>[7x]SMHTQSQTVTVDQQEILNRANEVEAPMADPPTDVPITPCELTAAKNAAQQLVLSADNMREYLAAGAKERQRLATSLRNAAKAYGEVDEEAATALDNDGEGTVQAESAGAVGGDSSAELTDTPRVATAGEPNFMDLKEAARKLETGDQGASLAHFADGWNTFNLTLQGDVKRFRGFDNWEGDAATACEASLDQQRQWILHMAKLSAAMAKQAQYVAQLHVWARR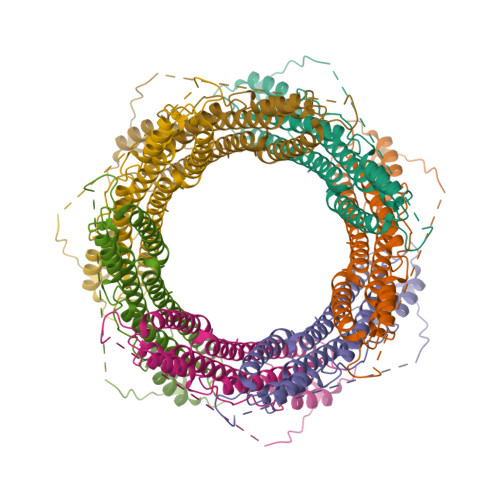EHPTYEDIVGLERLYAENPSARDQILPVYAEYQQRSEKVLTEYNNKAALEPVNPPKPPPAIKIDPP>MDRRRFLVGLLGLGLARGQGLRVEEVVGGLEVPWALAFLPDGGMLIAERPGRIRLFREGRLSTYAE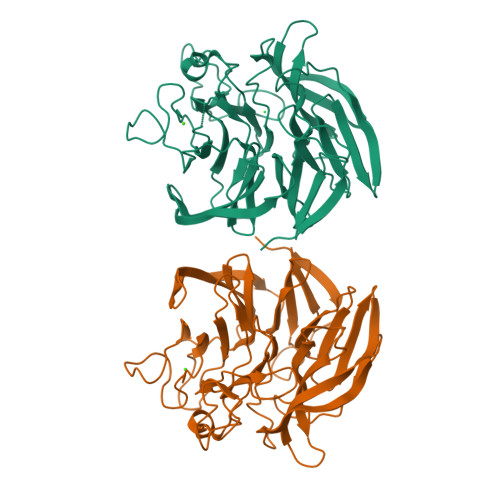LSVYHRGESGLLGLALHPRFPQEPYVYAYRTVAEGGLRNQVVRLRHLGERGVLDRVVLDGIPARPHGLHSGGRIAFGPDGMLYVTTGEVYERELAQDLASLGGKILRLTPEGEPAPGNPFLGRRGARPEVYSLGHRNPQGLAWHPKTGELFSSEHGPSGEQGYGHDEVNLIVPGGNYGWPRVVGRGNDPRYRDPLYFWPQGFPPGNLAFFRGDLYVAGLRGQALLRLVLEGERGRWRVLRVETALSGFGRLREVQVGPDGALYVTTSNRDGRGQVRPGDDRVLRLL[2x]> MASIDKQQIAASVPQRGFFGHPKGLFTLFFTEFWERFSYYGMRAILVYYMYYEVSKGGLGLDEHLALAIMSIYGALVYMSGIIGGWLADRVFGTSRAVFYGGLLIMAGHIALAIPGGVAALFVSMALIVLGTGLLKPNVSSIVGDMYKPGDDRRDAGFSIFYMGINLGAFLAPLVVGTAGMKYNFHLGFGLAAVGMFLGLVVFVATRKKNLGLAGTYVPNPL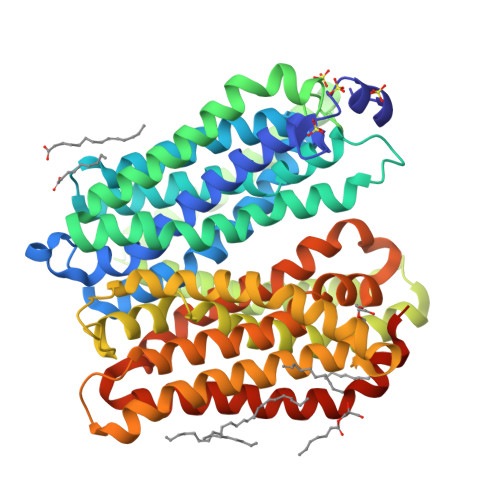TPAEKKKAAAIMAVGAVVIAVLLAILIPNGWFTVETFISLVGILGIIIPIIYFVVMYRSPKTTAEERSRVIAYIPLFVASAMFWAIQEQGSTILANYADKRTQLDVAGIHLSPAWFQSLNPLFIIILAPVFAWMWVKLGKRQPTIPQKFALGLLFAGLSFIVILVPGHLSGGGLVHPIWLVLSYFIVVLGELCLSPVGLSATTKLAPAAFSAQTMSLWFLSNAAAQAINAQLVRFYTPENETAYFGTIGGAALVLGLILLAIAPRIGRLMKGIRLESSGENLYFQ> MSTTSMTAPATSPSRLESMRAASSTTSSKPAPTGPSKKSDAPAKTKRQDKPNVNSANDSNAADTGTAAAATRPDHGRRSRRTEDANWLNAEKPGNAYRPADKELSQNVKVVQDDILNREQAQREQAERAQRQKEKLEQHISESPAGFQAALPRLNELDVANSWDKLLRMMRSEYDMSCLTSCLARELDEDVAWNPEMLLVQLTSDMLDAAELQKDSGEA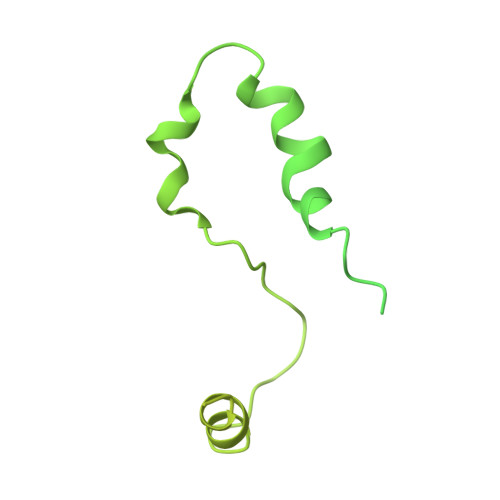YVPVDASDIGQMTGGEVARKRKAKRTKAAGGAEGEPEKDTEMPATASPPPTSQAATSKTPRKKATTDPAAAEPKKTQTGKAQNAGPTSAGNSSLPQKGSAAGSTSGAAGGGGGSKTSAAPSTAKRDASKDANATKSSSSKKKTSKQVSK>MDHAEENEILAATQRYYVERPIFSHPVLQERLHTKDKVPDSIADKLKQAFTCTPKKIRNIIYMFLPITKWLPAYKFKEYVLGDLVSGISTGVLQLPQGLAFAMLAAVPPIFGLYSSFYPVIMYCFLGTSRHISIGPFAVISLMIGGVAVRLVPDDIVIPGGVNATNGTEARDALRVKVAMSVTLLSGIIQFCLGVCRFGFVAIYLTEPLVRGFTTAAAVHVFTSMLKYLFGVKTKRYSGIFSVVYSTVAVLQNVKNLNVCSLGVGLMVFGLLLGGKEFNERFKEKLPAPIPLEFFAVVMGTGISAGFNLKESYNVDVVGTLPLGLLPPANPDTSLFHLVYVDAIAIAIVGFSVTISMAKTLANKHGYQVDGNQELIALGLCNSIGSLFQTFSISCSLSRSLVQEGTGGKTQLAGCLASLMILLVILATGFLFESLPQAVLSAIVIVNLKGMFMQFSDLPFFWRTSKIELTIWLTTFVSSLFLGLDYGLITAVIIALLTVIYRTQSPSYKVLGKLPETDVYIDIDAYEEVKE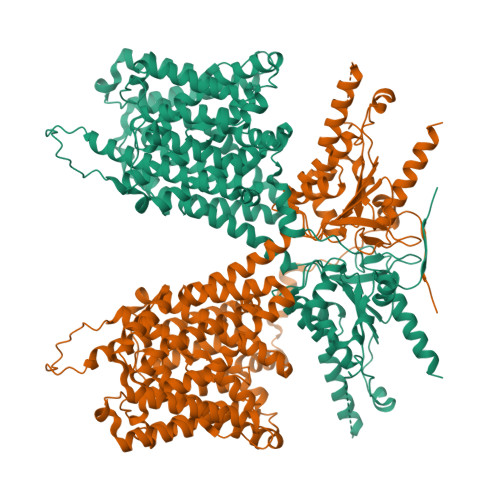IPGIKIFQINAPIYYANSDLYSNALKRKTGVNPAVIMGARRKAMRKYAKEVGNANMANATVVKADAEVDGEDATKPEEEDGEVKYPPIVIKSTFPEEMQRFMPPGDNVHTVILDFTQVNFIDSVGVKTLAGIVKEYGDVGIYVYLAGCSAQVVNDLTRNRFFENPALWELLFHSIHDAVLGSQLREALAEQEASAPPSQEDLEPNATPATPEALEVLFQ[2x]> MGAEKKLFLKALKE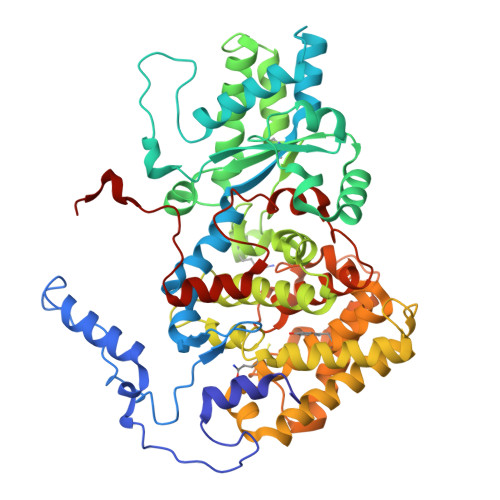KFEEDPKEKYTKFYVFGGWRQSARKREFVEAAEKLAEKRGGIPFYNPDIGVPLGQRKLMPYKLSGTDYIVEGDDLHFMNNAAMQQFWDDIRRTVIVGMDTAHAVLEKRLGVEVTPETINEYMETINHALPGGAVVQEHMVEVHPALAWDCYAKIFTGDDELADEIDKKFLIDINKLFPEEQAEQLKAAIGKRTYQVSRVPTLVGRVCDGGTIARWSAMQIGMSFITAYKLCAGEAAIADFSYAAKHADVIQMGTLLPARRARGPNEPGGIPFGILADVVQTTRVSDDPVEQSLEVVASGAMLYDQIWLGSYMSGGVGFTQYATASYTDDILDDFSYYGYDYVEKKYGICGAKPTMDVVEDIATEVTLYALECYDEFPALLEDHFGGSQRAAVAAAASGISVCMATGNSNAGLNGWYLSQILHKEYHSRLGFYGYDLQDQCGASNSLSIRNDESSPLELRGPNYPNYAMNVGHQGEYAGITQAAHSARKDAFALNPLIKVAFADPSLVFDFSHPRKEFARGALREFEPAGERDPIIPAH1lambda~6~,2-thiazetidine-1,1-dione 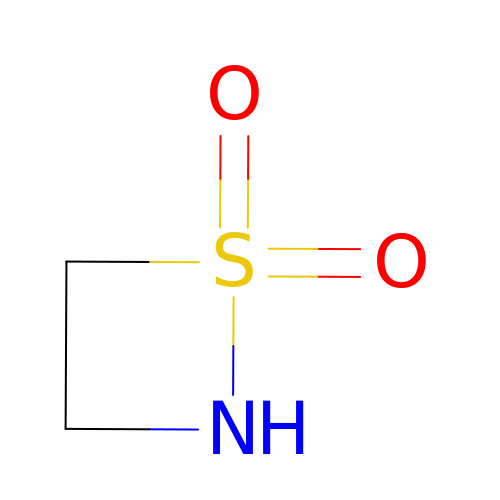| C2 H5 N O2 S | GNPXXOFTVXIOLF-UHFFFAOYSA-N>[6x]KLPTNLAYERSIDPSDVCFFVVWPDDRKTPLTYNSRTLLGQMEAKSLAYDVSGQPIKSATAEALAQGNPHQVDFCHVPYGASHIECSFSVSFSSELRQPYKCNSSKVKQTLVQLVELYETKIGWTELATRYLMNICNGKWLWKNTRKAYCWNIVLTPWPWNGEKVGFEDIRTNYTSRQDFKNNKNWSAIVEMIKTAFSSTDGLAIFEVRATLHLPTNAMVRPSQVFTEKEAAAAAAATQNSRVFQSTTIDGERSPILGAFKTGAAIATIDDWYPEATEPLRVGRFGVHREDVTCYRHPSTGKDFFSILQQAEHYIEVLSANKTPAQETINDMHFLMANLIKGGMFQHKGD;> LKELIASNPDDLTTELKRAFRPLTPHIAIDGNELDALTILVNLTDKTDDQKDLLDRAKCKQKLRDEKWWASCINCVNYRQSHNPKFPDIRSEGVIRTQALGELPSFLLSSSKIPPYHWSYSHDSKYVNKSAFLTNEFCWDGEISCLGELLKDADHPLWNTLKKLGCSQKTCKAMAKQLADITLTTINVTLAPNYLTQISLPDSDTSYISLSPVASLSMQSHFHQRLQD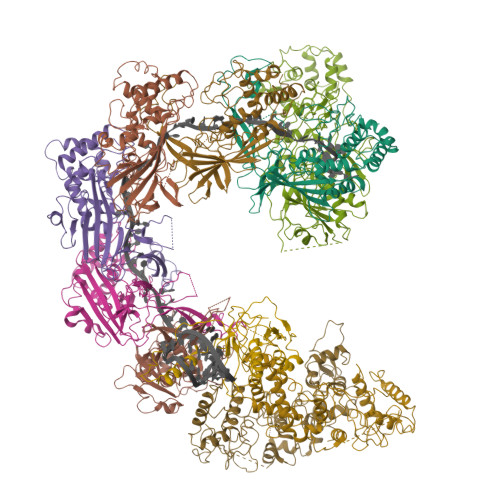ENRHSAITRFSRTTNMGVTAMTCGGAFRMLKSGAKFSSPPHHRLNNGSFLVLPNIRVCGATALSSPVTVGIPSLTAFFGFVHAFERNINRTTSSFRVESFAICVHQLHVEKRGLTAEFVEKGDGTISAPATRDDWQCDVVFSLILNTNFAQHIDQDTLVTSLPKRLARGSAKIAIDDFKHINSFSTLETAIESLPIEAGRWLSLYAQSNNNLSDLLAAMTEDHQLMASCVGYHLLEEPKDKPNSLRGYKHAIAECIIGLINSITFSSETDPNTIFWSLKNYQNYLVVQPRSIN;> KWYYKTITFLPELCNNESLAAKCLRVLHGFNYQYETRNIGVSFPLWCDATVGKKISFVSKNKIELDLLLKQHYFVQMEQLQYFHISNTVLVPEDCTYVSFRRCQSIDKLTAAGLARKIRRLEKRALSRGEQFDPSSFAQKEHTAIAHYHSLGESSKQTNRNFRLNIRMLSEQPREGNSIFSSYGLSNSENSFQPVPLI;> AMFLQRPKPYSDESLESFFIRVANKNGYGDVHRFLEATKRFLQDIDHNGYQTFPTDITRINPYSAKNSSSARTASFLKLAQLTFNEPPELLGLAINRTNMKYSPSTSAVVRGAEVFPRSLLRTHSIPCCPLCLRENGYASYLWHFQGYEYCHSHNVPLITTCSGHEAACTVSNWLAGHESKPLPNLPKSYRWGLVHWWMGIKDSDHFSFVQFFSNWPRSFHSIIEDEVEFNLEHAVVSTSELRLKDLLGRLFFGSIRLPERNLQHNIILGELLCYLENRLWQDKGLIANLKMNALEATVMLNCSLDQIASMVEQRILKPNRKSKDVTDYLFHFGDIFCLWLAEFQSDEFNRSFYVSRW;> AMFLQRPKPYSDESLESFFIRVANKNGYGDVHRFLEATKRFLQDIDHNGYQTFPTDITRINPYSAKNSSSARTASFLKLAQLTFNEPPELLGLAINRTNMKYSPSTSAVVRGAEVFPRSLLRTHSIPCCPLCLRENGYASYLWHFQGYEYCHSHNVPLITTCSCGKEFDYRVSEAACTVSNWLAGHESKPLPNLPKSYRWGLVHWWMGIKDDHFSFVQFFSNWPRSFHSIIEDEVEFNLEHAVVSTSELRLKDLLGRLFFGSIRLPERNLQHNIILGELLCYLENRLWQDKGLIANLKMNALEATVMLNCSLDQIASMVEQRILKPNAAAAAAAAADVTDYLFHFGDIFCLWLAEFQSDEFNRSFYVSR>[3x]MKRDLLAIQAVRAMDDIDKTINLFSERLREWYSIHFPELDKLIEDHEEYATIVSRFGDRGFLTIDSLKELGFNEQRINRI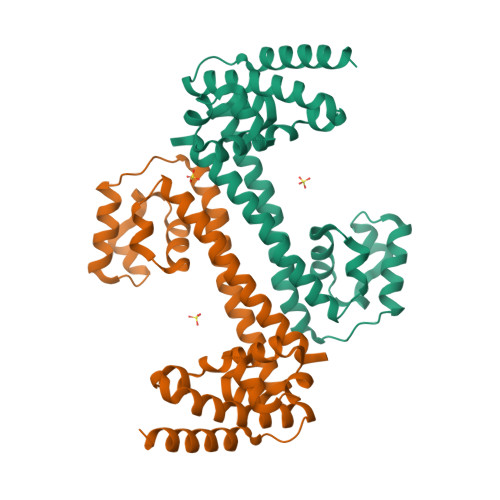LDAAKKSIGADISEDDLSAMRMIANTILDLYNIRRNLNNYLEGVMKEVAPNVTALVGPALGARLLSIAGSLDELAKMPASTIQVLGAEKALFRALRSGGRPPKHGIIFQYPAIHTSPRWQRGKIARALAAKLAIAARVDAFSGRFIGDQLNEQLKKRIDEIKEKFAQHHHHHHHH> N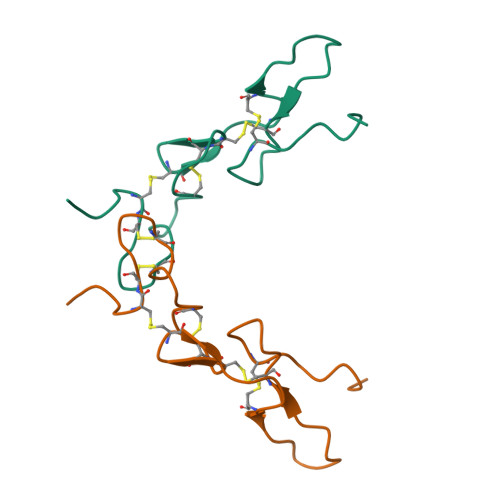SVHPCCDPVICEPREGEHCISGPCCENCYFLNSGTICKRARGDGNQDYCTGITPDCPRNRYNV L-gamma-glutamyl-S-nonyl-L-cysteinylglycine | C19 H35 N3 O6 S | 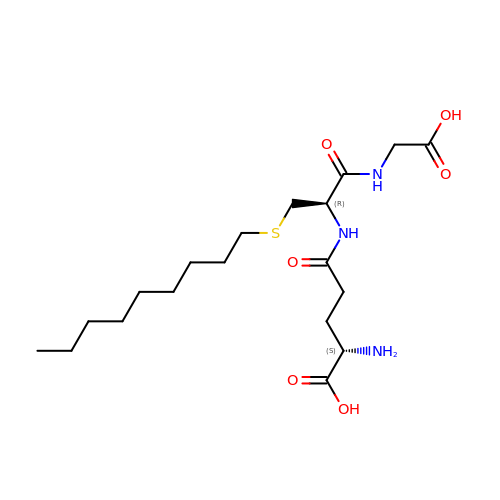LUOWFOMONLCPJP-GJZGRUSLSA-N>MALKAQNTISGKEGRLFLDGEEMAHIKTF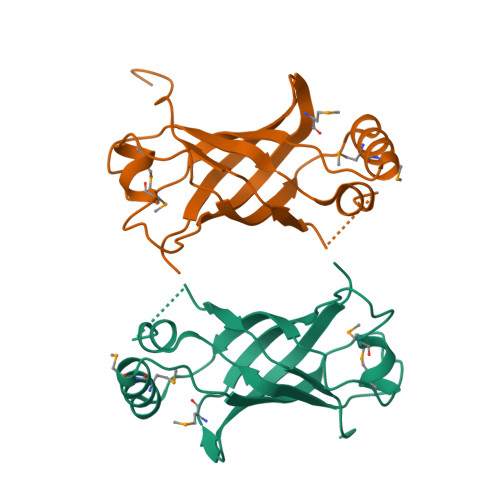EANVEKNKSEVNIMGRRMTGHKTTGANGTGTATFYKVTSKFVLLMMDYVKKGSDPYFTLQAVLDDQSSGRGTERVTLYDVNFDSAKIASLDVDSEALEEEVPFTFEDFDVPEKLSDTFLEHHHHHH[2x]> AQNNPYLFRSNKFLTLFKNQHGSLRLLQRFNEDTEKLENLRDYRVLEYCSKPNTLLLPHHSDSDLLVLVLEGQAILVLVNPDGRDTYKLDQGDAIKIQAGTPFYLINPDNNQNLRILKFAITFRRPGTVEDFFLSSTKRLPSYLSAFSKNFLEASYDSPYDEIEQTLLQEEQEGVIVKM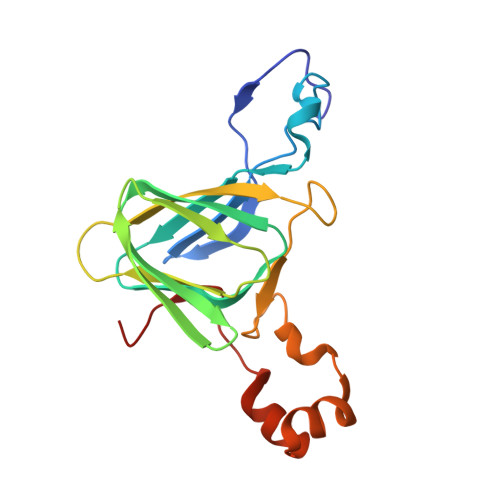PK>REWFLHRNSLIVLADVALFLALYHFLPFEHNVVLGISMLAFIAVLWLTEALHVTVTAILVPVMAVFFGIFETQAALNNFANSIIFLFLGGFALAAAMHHQGLDKVIADKVLAMAQGKMSVAVFMLFGVTALLSMWISNTATAAMMLPLVLGVLSKVDADKQRSTYVFVLLGVAYSASIGGIATLVGSPPNAIAAAEVGLSFTDWMKFGLPTAMMMLPMAIAILYFLLKPTLNGMFELDRAPVNWDKGKVVTLGIFGLTVFLWIFSSPINAALGGFKSFDTLVALGAILMLSFARVVHWKEIQKTADWGVLLLFGGGLCLSNVLKQTGTSVFLANALSDMVSHMGIFVVILVVATFVVFLTEFASNTASAALLIPVFATVAEAFGMSPVLLSVLIAVAASCAFMLPVATPPNAIVFASGHIKQSEMMRVGLYLNIA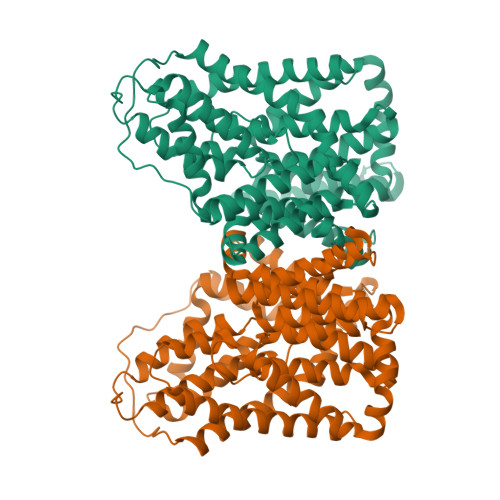CIGLLTAIAMLFWQ[2x]> GGAUGUACUACCAGCUGAUGAGUCCCAA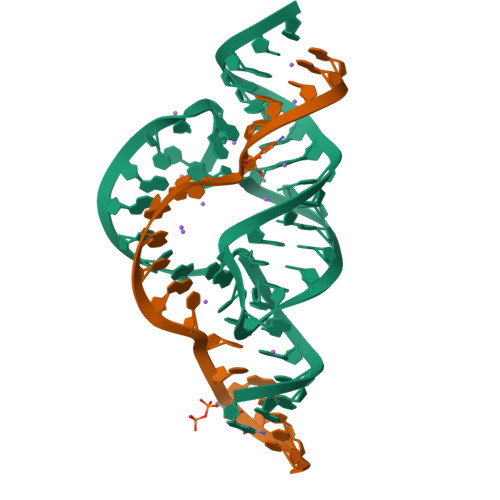AUAGGACGAAACGCC;> GGCGUCCUGGUAUCCAAUCC>[2x]MHHHHHHEGELKTILGQAKVSKLQEKLKLDPRSKITFNDFKGIAK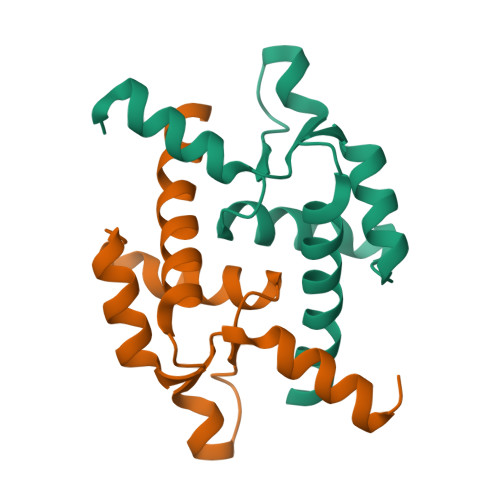EVGIEEKEINSVSNALAQSGSIIYLPNSLNENLKTSVFTKPAHIYQSLEHILDIENKGVG> MELKHSISDYTEAEFLQLVTTICNADTSSEEELVKLVTHFEEMTEHPSGSDLIYFPKEGDDDSPSGIVNTVKQWRAANGKSGFKQG;> MESKRNKPGKATGKGKPVGDKWLDDAGKDSGAPIPDRIADKLRDKEFKSFDD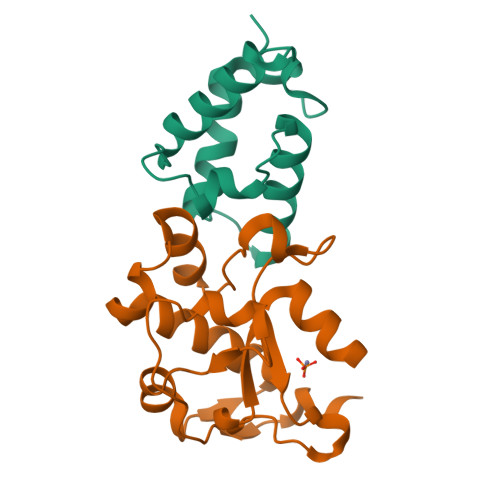FRKAVWEEVSKDPELSKNLNPSNKSSVSKGYSPFTPKNQQVGGRKVYELHHDKPISQGGEVYDMDNIRVTTPKRHIDIHRGK Here we reveal that two atypical acyl-CoA dehydrogenases, ACAD10 and ACAD11, drive 4-HA catabolism in mice. Unlike other ACADs, ACAD10 and ACAD11 feature kinase domains that phosphorylate the 4-hydroxy position as a requisite step in converting 4-hydroxyacyl-CoAs into conventional 2-enoyl-CoAs. ACAD10/11 are evolutionarily divergent members of the ACAD family, possessing both an N-terminal kinase domain and unconventional hydrophilic residues in the ACAD active site. These features allow them to phosphorylate and process 4-hydroxylated acyl-CoA substrates, ultimately removing the hydroxy group and producing 2-enoyl-CoAs that can enter the FAO cycle.

In the first mutant (K*), we replaced the catalytic aspartate of the kinase domain with alanine, thereby eliminating kinase activity but leaving ACAD activity intact. To further explore the bifunctionality of ACAD10/11 at the molecular level, we initiated cryo-electron microscopy (cryo-EM) experiments with the ACAD11 K* and A* mutant proteins purified from Escherichia coli. To assess whether substrate interactions affect protein structure, these mutants were incubated with 4-HV-CoA and 4-PV-CoA, respectively, before preparation. Analysis of the ACAD11 K* mutant particles revealed an intact, tetrameric structure but only the ACAD domains were resolved. The active sites of the tetrameric ACAD domain show density that is consistent with bound flavin adenine dinucleotide (FAD). The K* mutants demonstrated little to no substrate consumption, whereas the A* mutants generated the 4-PV-CoA intermediate but were unable to complete conversion into 2-pentenoyl-CoA.

>[4x]ETDVTSDTVEVLPQHKFDLRSLEAYLNQHLPGFGSDSRAVLTVTQYRSGQSNPTFFLQKGSQAYVLRKKPPGSLLPKAHKIDREFKIQKALFSIGFPVAKPLLYCRDASVIGTEFYVMEHVQGRIFRDFSIPGVSSAERAAIYVSVAETLAWLHSLDIRSLKLDKYGTGVGYCKRQVSTWTKQYQASAHQSIPAMDQLSTWLMKNLPDSDSEECLVHGAFKLDNIVFHPKECRVIAVLDWELSTFGHPLTDLAHLSLFYYWPRTLPMINRGSHIPENTGIPLMEELISIYCHRRGIDPNLPNWNFFMALSFFKLAGISQGVYRRYLMGNNSSEDSFLTANTVQPLAETGLQLSKRTLRTTPPQADAKSQLFAQSRRGQEVLTRVKQFMKQHVFPAEKEVAEYYAQSGNSAEKWGHPLVIEKLKEIAKAEGLWNLFLPAVSGLSQVDYALIAEETGKCFFAPDVFNCQAPDTGNMEVLHLYGSEQQKKQWLEPLLRGDITSVFCMTEPNVSSSDATNIECTIQRDGGGYIVNGKKWWSSGAGNPKCKIAIVLGRTESPSASRHRQHSMILVPMDTPGVELIRPLSVFGYMDNMHGGHWEVHFNHVRVPASNLILGEGRGFEISQGRLGPGRIHHCMRTVGLAERILQIMCDRAVQREAFKKKLYEHEVVAHWIAKSRIAIEEIRLLTLKAAHSIDTLGSASARKEIAMIKVAAPKAVCKIADWAIQVHGGAGVSQDYPLANMYAIIRTLRLADGPDEVHLSAIAKMELQDQARRLTARM>GHMNAAPNRNLFDRVLHGQAPCFALIARSTGSAGERAMIDVFAGAVSYPSSLAELPLAAPTATGADRQELLVMVPYRQLHERGFKTHDDGAPLVAITCDEHETVSAQLALAAIPDADTALGERHFDIDDEAYAEIVERVITDEIGTGAGSNFVIKRTLEGDLDDYSPAKALAVFKRLMRREVGAYWIFVIHTGERTFVGATPERHLTLHEGCATMNPISGTYRYPQSGPTIDGINAFLGDRKESDELYMVLDEELKMMARICPAGGQVTGPHLREMARLAHTEYFIVGHTEADVRDLLRETMFAPTVTGSPIESATRVIARHERAGRGYYSGIAALIGRDARGGRTLDSAILIRTAEIDRAGHVRIGVGSTLVRHSDAVSEVMETHAKVAALSNAFDPPEAGPALGQHPSVQAALRERNEGIADFWFRPYGGRQGEMADELAELSGCRALIVDAEDHFTAMIAQQLSSLGLATEVCGVHDAVDLARYDVVVMGPGPGDPSDAGDPRIARLYAWLRHLIDEGKPFMAVCLSHQILNA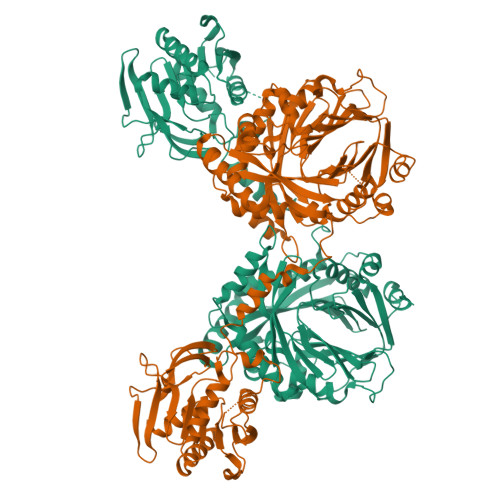ILGIPLVRREVPNQGIQVEIDLFGQRERVGFYNTYVAQTVRDEMDVDGVGTVAISRDPRTGEVHALRGPTFSSMQFHAESVLTVDGPRILGEAITHAIRREKRMTALTA[2x]2-deoxy-2-fluoro-1-O-[(S)-hydroxy{[(2E,6E)-3,7,11-trimethyldodeca-2,6,10-trien-1-yl]oxy}phosphoryl]-beta-D-arabinofuranose 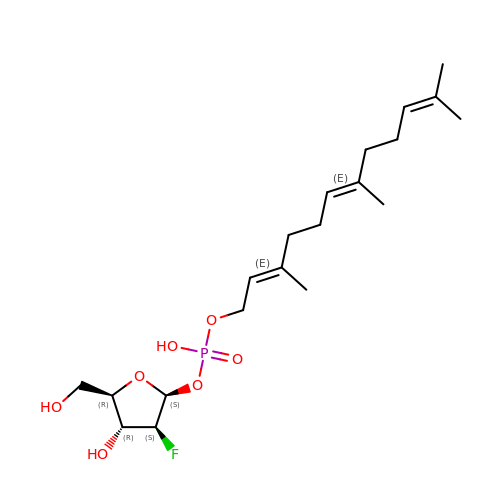| C20 H34 F O7 P | UVMYWRMMMKEFCL-KTRXZIFQSA-N> MERYENLFAQLNDRREGAFVPFVTLGDPGIEQSLKIIDTLIDAGADALELGVPFSDPLADGPTIQNANLRAFAAGVTP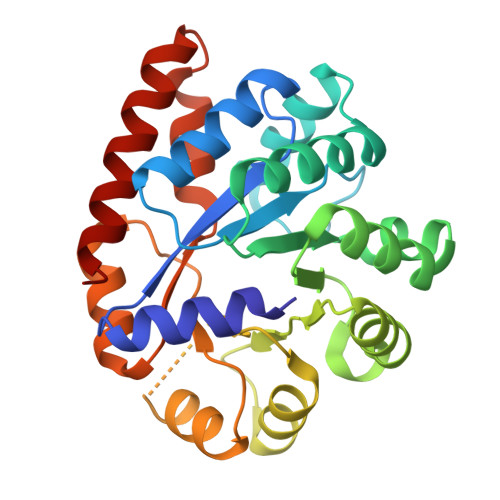AQCFEMLALIREKHPTIPIGLLMYANLVFNNGIDAFYARCEQVGVDSVLVADVPVEESAPFRQAALRHNIAPIFICPPNADDDLLRQVASYGRGYTYLLSRSGVVGAENRGALPLHHLIEKLKEYHAAPALQGFGISSPEQVSAAVRAGAAGAISGSAIVKIIEKNLASPKQMLAELRSFVSAMKAASRA>SEGSDAPNFVLEDTNGKRIELSDLKGKGVFLNFWGTWCEPAKKEFPYMANQYKHFKSQGVEIVAVNVGESKIAVHNFMKSYGVNFPVVLDTDRQVLDAYDVSPLPTTFLINPEGKVVKVVTGTMTES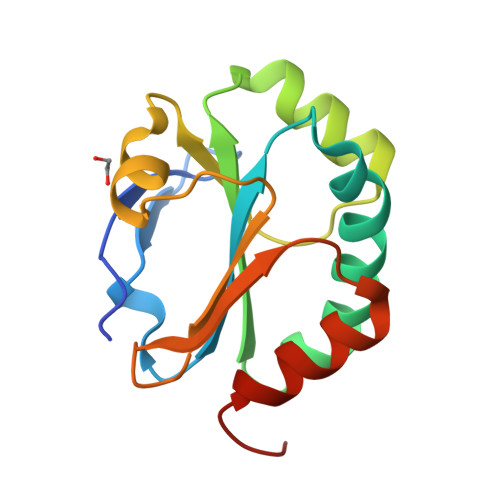MIHDYMNLIKPGETSG[2x]> MTEGAKKAPVIWVQGQGCTGCSVSLLNAVHPRIKEILLDVISLEFHPTVMASEGEMALAHMYEIAEKFNGNFFLLVEGAIPTAKEGRYCIVGETLDAKAHHHEVTMMELIRDLAPKSLATVAVGTCSAYGGIPAAEGNVTGSKSVRDFFADEKIEKLLVNVPGCPPHPDWMVGTLVAAWSHVLNPTEHPLPELDDDGR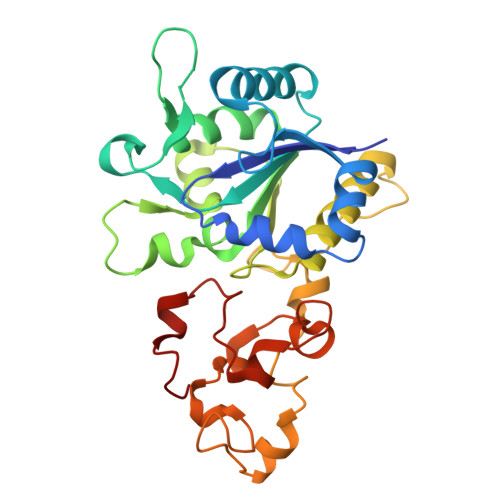PLLFFGDNIHENCPYLDKYDNSEFAETFTKPGCKAELGCKGPSTYADCAKRRWNNGINWCVENAVCIGCVEPDFPDGKSPFYVAE> MSELKDIIAAVTPCKGADFELQALKIRQPQGDEVLVKVVATGMCHTDLIVRDQKYPVPLPAVLGHEGSGIIEAIGPNVTELQVGDHVVLSYGYCGKCTQCNTGNPAYCSEFFGRNFSGADSEGNHALCTHDQGVVNDHFFAQSS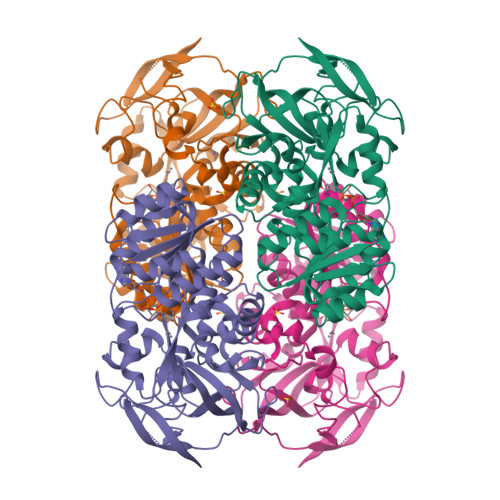FATYALSRENNTVKVTKDVPIELLGPLGCGIQTGAGACINALKVTPASSFVTWGAGAVGLSALLAAKVCGASIIIAVDIVESRLELAKQLGATHVINSKTQDPVAAIKEITDGGVNFALESTGSPEILKQGVDALGILGKIAVVGAPQLGTTAQFDVNDLLLGGKTILGVVEGSGSPKKFIPELVRLYQQGKFPFDQLVKFYAFDEINQAAIDSRKGITLKPIIKIA> MTVKAPSVTSLRISKLSANQVQVRWDDVGANFYYFVEIAETKTNSGENLPSNQYRWINLGYTANNSFFFDDADPLTTYIIRVATAAQDFEQSDWIYTEEFETFATNAYTFQNMIEMQLANKFIQEKFTLNNSDYVNFNNDTIMAALMNESFQFSP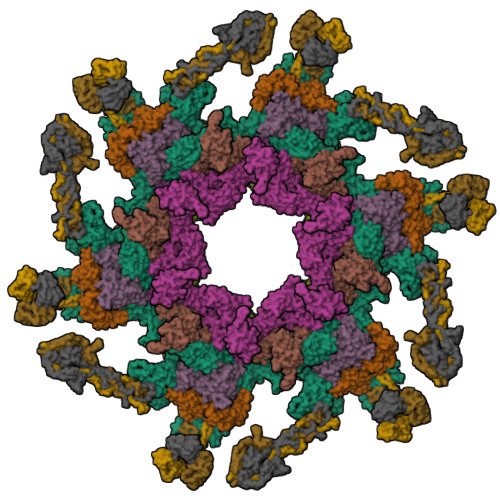SYVDVSSISNFIIGENEYHEIQGSIQQVCKDINRVYLMESEGILYLFERYQPVVKVSNDKGQTWKAVKLFNDRVGYPLSKTVYYQSANTTYVLGYDKIFYGRKSTDVRWSADDVRFSSQDITFAKLGDQLHLGFDVEIFATYATLPANVYRIAEAITCTDDYIYVVARDKVRYIKTSNALIDFDPLSPTYSERLFEPDTMTITGNPKAVCYKMDSICDKVFALIIGEVETLNANPRTSKIIDSADKGIYVLNHDEKTWKRVFGNTEEERRRIQPGYANMSTDGKLVSLSSSNFKFLSDNVVNDPETAAKYQLIGAVKYEFPREWLADKHYHMMAFIADETSDWETFTPQPMKYYAEPFFNWSKKSNTRCWINNSDRAVVVYADLKYTKVIENIPETSPDRLVHEYWDDGDCTIVMPNVKFTGFKKYASGMLFYKASGEIISYYDFNYRVRDTVEIIWKPTEVFLKAFLQNQEHETPWSPEEERGLADPDLRPLIGTMMPDSYLLQDSNFEAFCEAYIQYLSDGYGTQYNNLRNLIRNQYPREEHAWEYLWSEIYKRNIYLNADKRDAVARFFESRSYDFYSTKGIEASYKFLFKVLYNEEVEIEIESGAGTEYDIIVQSDSLTEDLVGQTIYTATGRCNVTYIERSYSNGKLQWTVTIHNLLGRLIAGQEVKAERLPSFEGEIIRGVKGKDLLQNNIDYINRSRSYYVMKIKSNLPSSRWKSDVIRFVHPVGFGFIAITLLTMFINVGLTLKHTETIINKYKNYKWDSGLPTEYADRIAKLTPTGEIEHDSVTGEAIYEPGPMAGVKYPLPDDYNAENNNSIFQGQLPSERRKLMSPLFDASGTTFAQFRDLVNKRLKDNIGNPRDPENPTQVKIDE;>[2x]MNDSSVIYRAIVTSKFRTEKMLNFYNSIGSGPDKNTIFITFGRSEPWSSNENEVGFAPPYPTDSVLGVTDMWTHMMGTVKVLPSMLDAVIPRRDWGDTRYPDPYTFRINDIVVCNSAPYNATESGAGWLVYRCLDVPDTGMCSIASLTDKDECLKLGGKWTPSARSMTPPEGRGDAEGTIEPGDGYVWEYLFEIPPDVSINRCTNEYIVVPWPEELKEDPTRWGYEDNLTWQQDDFGLIYRVKANTIRFKAYLDSVYFPEAALPGNKGFRQISIITNPLEAKAHPNDPNVKAEKDYYDPEDLMRHSGEMIYMENRPPIIMAMDQTEEINILFTF;>[2x]MANTPVNYQLTRTANAIPEIFVGGTFAEIKQNLIEWLNGQNEFLDYDFEGSRLNVLCDLLAYNTLYIQQFGNAAVYESFMRTANLRSSVVQAAQDNGYLPTSKSAAQTEIMLTCTDALNRNYITIPRGTRFLAYAKDTSVNPYNFVSREDVIAIRDKNNQYFPRLKLAQGRIVRTEIIYDKLTPIIIYDKNIDRNQVKLYVDGAEWINWTRKSMVHAGSTSTIYYMRETIDGNTEFYFGEGEISVNASEGALTANYIGGLKPTQNSTIVIEYISTNGADANGAVGFSYADTLTNITVININENPNDDPDFVGADGGGDPEDIERIRELGTIKRETQQRCVTATDYDTFVSERFGSIIQAVQTFTDSTKPGYAFIAAKPKSGLYLTTVQREDIKNYLKDYNLAPITPSIISPNYLFIKTNLKVTYALNKLQESEQWLEGQIIDKIDRYYTEDVEIFNSSFAKSKMLTYVDDADHSVIGSSATIQMVREVQNFYKTPEAGIKYNNQIKDRSMESNTFSFNSGRKVVNPDTGLEEDVLYDVRIVSTDRDSKGIGKVIIGPFASGDVTENENIQPYTGNDFNKLANSDGRDKYYVIGEINYPADVIYWNIAKINLTSEKFEVQTIELYSDPTDDVIFTRDGSLIVFENDLRPQYLTIDLEPISQ;> MLFTFFDPIEYAAKTVNKNAPTIPMTDIFRNYKDYFKRALAGYRLRTYYIKGSPRPEELANAIYGNPQLYWVLLMCNDNYDPYYGWITSQEAAYQASIQKYKNVGGDQIVYHVNENGEKFYNLISYDDNPYVWYDKGDKARKYPQYEGALAAVDTYEAAVLENEKLRQIKIIAKSDINSFMNDLIRIMEKSYGNDK;>[3x]MKQNINIGNVVDDGTGDYLRKGGIKINENFDELYYELGDGDVPYSAGAWKTYNASSGQTLTAEWGKSYAINTSSGRVTINLPKGTVNDYNKVIRARDVFATWNVNPVTLVAASGDTIKGSAVPVEINVRFSDLELVYCAPGRWEYVKNKQIDKITSSDISNVARKEFLVEVQGQTDFLDVFRGTSYNVNNIRVKHRGNELYYGDVFSENSDFGSPGENEGELVPLDGFNIRLRQPCNIGDTVQIETFMDGVSQWRSSYTRRQIRLLDSKLTSKTSLEGSIYVTDLSTMKSIPFSAFGLIPGEPINPNSLEVRFNGILQELAGTVGMPLFHCVGADSDDEVECSVLGGTWEQSHTDYSVETDENGIPEILHFDSVFEHGDIINITWFNNDLGTLLTKDEIIDETDNLYVSQGPGVDISGDVNLTDFDKIGWPNVEAVQSYQRAFNAVSNIFDTIYPIGTIYENAVNPNNPVTYMGFGSWKLFGQGKVLVGWNEDISDPNFALNNNDLDSGGNPSHTAGGTGGSTSVTLENANLPATETDEEVLIVDENGSVIVGGCQYDPDESGPIYTKYREAKASTNSTHTPPTSITNIQPYITVYRWIRIA> MGSDKIHHHHHHVKIAIASDHAAFELKEKVKNYLLGKGIEVEDHGTYSEESVDYPDYAKKVVQSILSNEADFGILLCGTGLGMSIAANRYRGIRAALCLFPDMARLARSHNNANILVLPGRLIGAEL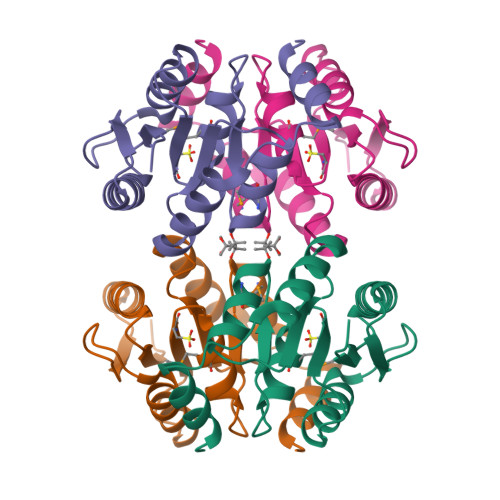AFWIVDTFLSTPFDGGRHERRIRKIDEV> GAMGSSKFEEFMTRHQVHEKEEFKALKTLSIFYQAGTSKAGNPIFYYVARRFKTGQINGDLLIYHVLLTLKPYYAKPYEIVVDLTHTGPSNRFKTDFLSKWFVVFPGFAYDNVSAVYIYNCNSWVREYTKYHERLLTGLKGSKRLVFIDCPGKLAEHIEHEQQKLPAATLALGHEQQKLPAATLALEEDLKVFHNALKLAHKDTKVSIKV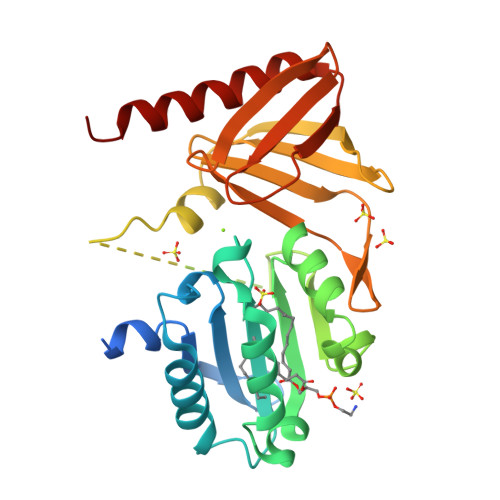GSTAVQVTSAERTKVLGQSVFLNDIYYASEIEEICLVDENQFTLTIANQGTPLTFMHQECEAIVQSIIHIRTRWELSQPD>[2x]MMANRMILNETAWFGRGAVGALTDEVKRRGYQKALIVTDKTLVQCGVVAKVTDKMDAAGLAWAIYDGVVPNPTITVVKEGLGVFQNSGADYLIAIGGGSPQDTCKAIGIIS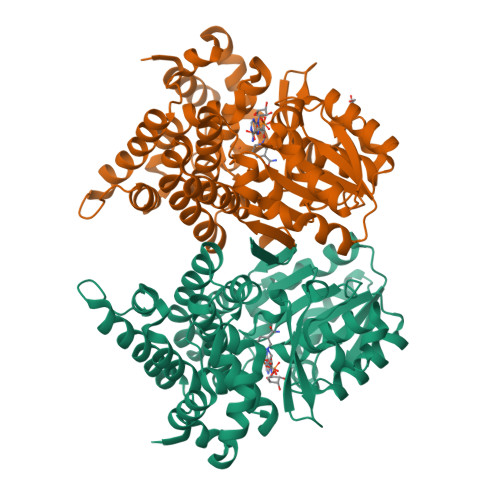NNPEFADVRSLEGLSPTNKPSVPILAIPTTAGTAAEVTIGYVITDEEKRRKFVCVDPHDIPQVAFIDADMMDGMPPALKAATGVDALTHAIEGYITRGAWALTDALHIKAIEIIAGALRGSVAGDKDAGEEMALGQYVAGMGFSNVGVGLVHGMAHPLGAFYNTPHGVANAILLPHVMRYNADFTGEKYRDIARVMGVKVEGMGLEEARNAAVEAVFALNRDVGIPPHLRDVGVRKEDIPALAQAALDDVCTGGNPREATLEDIVELYHTAWTSHHHHH> SNEWIQPRLPQ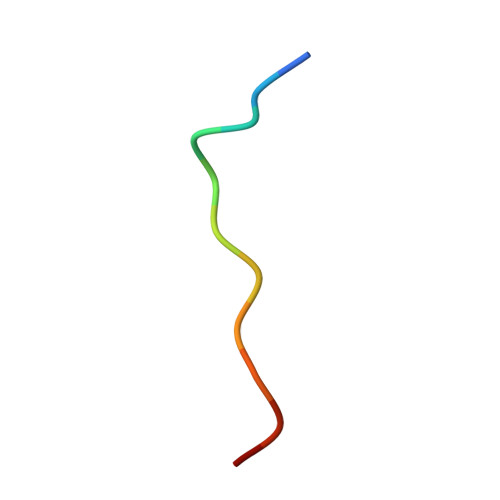H>MSQYSIQQSLGNASGVAVSPINADATLSTGVALNSSLWAGIGVFARGKPFTVLAVTESNYEDVLGEPLKPSSGSQFEPIRHVYEAIQQTSGYVVRAVPDDAKFPIIMFDESGEPAYSALPYGSEIELDSGEAFAIYVDDGDPCISPTRELTIETATADSAGNERFLLKLTQTTSLGVVTTLETHTVSLAEEAKDDMGRLCYLPTALEARSKYLRAVVNEELISTAKVTNKKSLAFTGGTNGDQSKISTAAYLRAVKVLNNAPYMYTAVLGLGCYDNAAITALGKICADRLIDGFFDVKPTLTYAEALPAVEDTGLLGTDYVSCSVYHYPFSCKDKWTQSRVVFGLSGVAYAAKARGVKKNSDVGGWHYSPAGEERAVIARASIQPLYPEDTPDEEAMVKGRLNKVSVGTSGQMIIDDALTCCTQDNYLHFQHVPSLMNAISRFFVQLARQMKHSPDGITAAGLTKGMTKLLDRF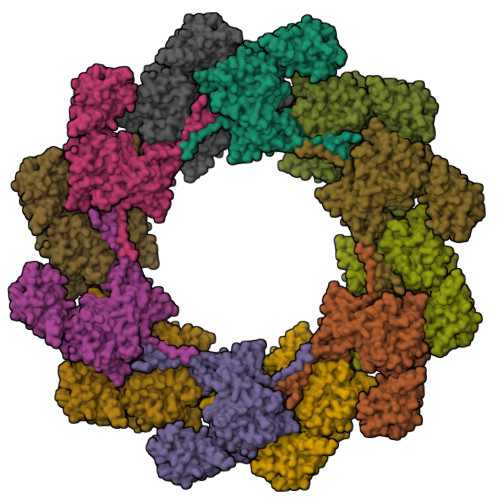VASGALVAPRDPDADGTEPYVLKVTQAEFDKWEVVWACCPTGVARRIQGVPLLIK[12x]> MGSSHHHHHHSQDPMEIDELTALGGLLHDIGKPVQRAGLYSGDHSTQGARFLRDLAENTGRAEYELLSLFSEFHHKGHMKNDELMIRRIKELSPERFGLTMEDVLNALWIVYEADNLASGEREEGQPQASRPLYSVFNPGKAYPWAELDFEKELPVPGDVFSIRSQDYRELVKRLWEELSKAKLRSDRLLPVLEKYLTFVSSVTSEGNIISLYDHMRMTSAIALAMLRAGCTAEDVRSGRCRKEKRFLLIEGDFSGIQDFIYRVSGKGTLKYLRARSAYLELIGWDVVLEILSRLGLTRANVVFNAGGHFMIIAQNTPDAVKELEEIRAKAVEWLYREFESDLYLAIEWEPVSGREFGREGGKNLFAEARKRLKHKLTVRKLKRFGEIKGLFEHGHTERLAECPVCGRELPEGKLEPSASDPETKVCPTCNRLVSLGGNLPKLLGFGRTAKNDAGVLVEGPFSGFVPYLQGGRPVGEQILVKNTLNPGEIPESAQFVPYFVADYFKKDPKGGVATFEELSMASTGTRRLGVMKGDVDRLGEFFSSMDSPSKLATASRFMDYFFKGYIGAIIEGKFGYIIGDVPSLRDWPEEPDIVVVYAGGDDFFIVGAWDQIFELAFRVRRAFNAYTGGKLTLSVGLGYFDERTPIYRMADVVSERLDTAKDEGRNRVFVVGRSRP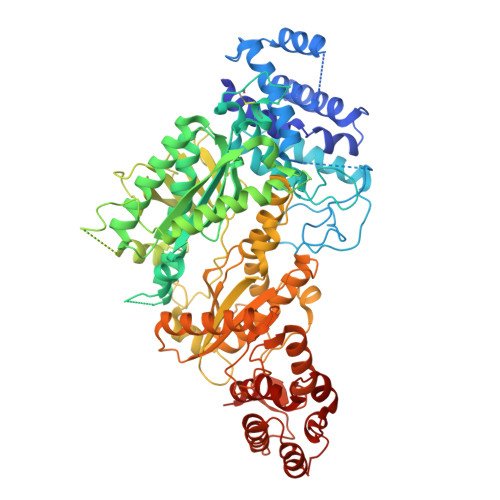LDGKHKLSYEWNHYEELWRTYAPRIYAGNGRLKGKLESKKGLLWKLLEIRELYVRDPNDVRWAYLTAYLLGRHGLSDLFPELVGIDTKAVERKEPQPVYWVDGVLKIVLMAVRR> MIFPKQYP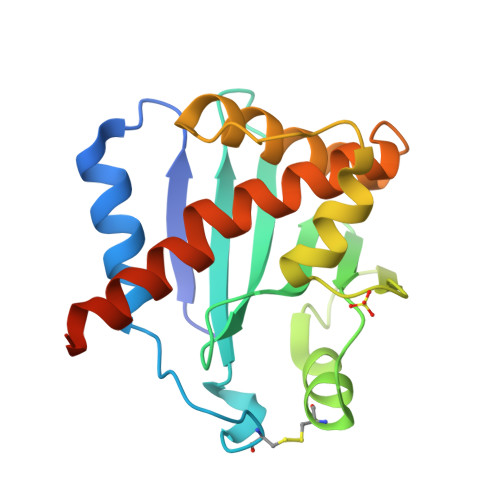IINFTTAGATVQSYTNFIRAVRGRLTVLPNRCGLPINQRFILVELSNHAELSVTLALDVTNAYVVGYRAGNSAYFFHPDNQCDAEAITHLFTDVQNRYTFAFGGNYDRLEQLAGNLRENIELGNGPLEEAISALYYYSTGGTQLPTLARSFIICIQMISEAARFQYIEGEMRTRIRYNRRS>[2x]MIRMRTPSTLPFTKMHGAGNDFVVLDLRDGPDPSPELCRALADRHKGVGCDLVLGIREPRSARAVAAFDIWTADGSRSAQCGNGARCVAAWAVRAGLARGPRFALDSPSGTHEVDVLDADTFRVALAV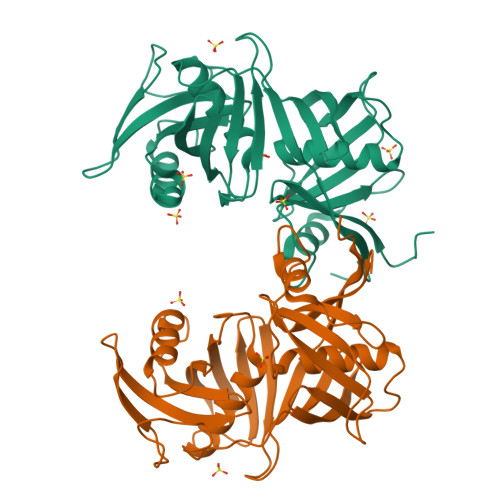PRFAPESIPLFGHDGEQDLYEADLGDGTRVRFAAVSMGNPHAVIEVDDTATAPVARVGRAVQASGLFLPTVNVGFARVESRDRVHLRVHEYGAGETLACGSGACAAAAVLMRRGRVDRNVSVVLPGGELRISWPDDAADVLMTGPAAFVYEGTFLHASVLEHHHHHH>MTLYSKKDIVQQARNLAKMISETEEVDFFKRAEAQINENDKVSTIVNQIKALQKQAVNLKHYEKHEALKQVEAKIDALQEELEEIPVIQEFRDSQMEVNDLLQLVAHTISNQVTNEIITSTGGDLLKGETGSKVKHSNNSCSL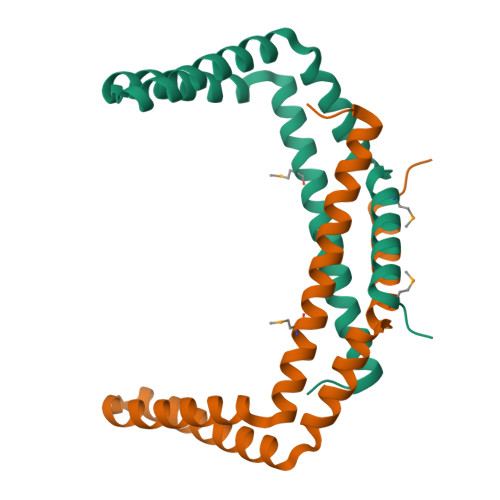LEHHHHHH[2x]> KKKLPA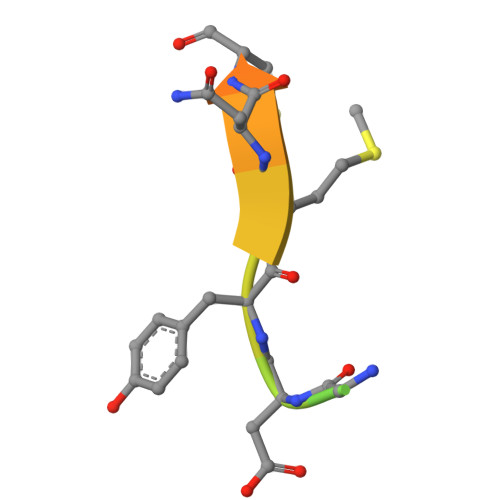TGDYMNMSPVGD> ATLKDITRRLKSIKNIQKITKSMKMVAAAKYARAERELKPARVYGVGSLALYEKADIKTPEDKKKHLIIGVSSDRGLCGAIHSSVAKQMKSEAANLAAAGKEVKIIGVGDKIRSILHRTHSDQFLVTFKEVGRRPPTFGDASVIALELLNSGYEFDEGSIIFNRFRSVISYKTEEKPIFSLDTISSAESMSIYDDIDADVLRNYQEYSLANIIYYSLKESTTSEQSARMTAMDNASKNASEMIDKLTLTFNRTRQAVITKELIEIISGAAALD;> AEAAAAQAPAAGPGQMSFTFASPTQVFFNSANVRQVDVPTQTGAFGILAAHVPTLQVLRPGLVVVHAEDGTTSKYFVSSGSVTVNADSSVQLLAEEAVTLDMLDLGAAKANLEKAQSELLGAADEATRAEIQIRIEANEALVKALE;> VAYWRQAGL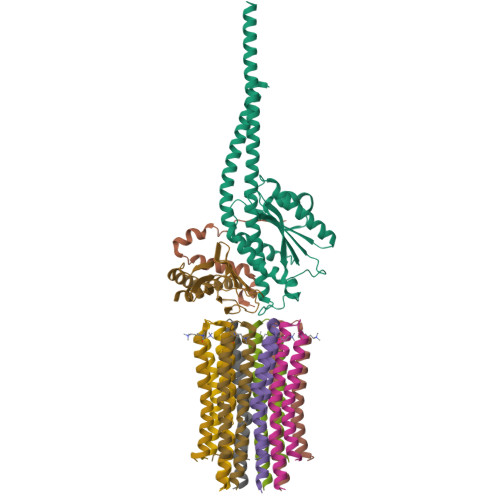SYIRYSQICAKAVRDALKTEFKANAMKTSGSTIKIVKVKKE;>DIDTAAKFIGAGAATVGVAGSGAGIGTVFGSLIIGYARNPSLKQQLFSYAILGFALSEAMGLFCLMVAFLILFAM[8x]>[4x]MQGSVTEFLKPRLVDIEQVSSTHAKVTLEPLERGFGHTLGNALRAILLSSMPGCAVTEVEIDGVLHEYSTKEGVQEDILEILLNLKGLAVRVQGKDEVILTLNKSGIGPVTAADITHDG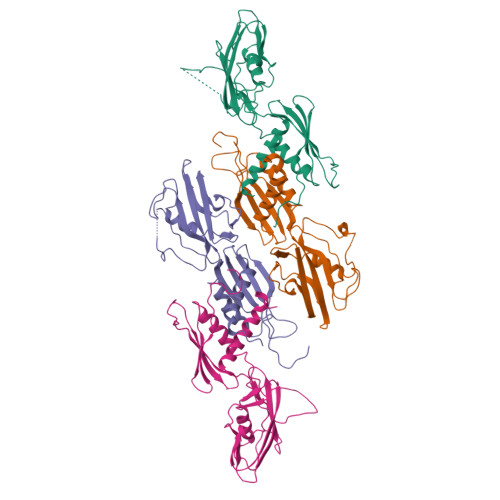DVEIVKPQHVICHLTDENASISMRIKVQRGRGYVPASTRIHSEEDERPIGRLLVDACYSPVERIAYNVEAARVEQRTDLDKLVIEMETNGTIDPEEAIRRAATILAEQLEAFVDLR>SMLKLSAENESTPIQQLLEHFLRQLQRKDPHGFFAFPVTDAIAPGYSMIIKHPMDFGTMKDKIVANEYKSVTEFKADFKLMCDNAMTYNRPDTVYYKLAKKILHAGFKMMSKERLLALKRSMS[2x]

Bromodomains (BRDs) are acetyl-lysine–dependent protein interaction modules that play a pivotal role in chromatin biology and control of gene expression. Acetyl-lysine recognition is mediated by a binding cleft formed by four canonical helices (αZ, αA, αB, and αC) and two connecting loop regions (ZA and BC loops). This interaction site is highly druggable, enabling the development of potent protein interaction inhibitors. To address this issue, we developed a promiscuous BRD inhibitor [bromosporine (BSP)] that broadly targets BRDs (including BETs) with nanomolar affinity, creating a tool for the identification of cellular processes and diseases where BRDs have a regulatory function.

To ascertain the predicted promiscuous binding mode, we determined high-resolution crystal structures with different human BRDs. In all cases, BSP was resolved well in the high-resolution structures and inserted into the acetyl-lysine binding cavity of each BRD module. In all cases, BSP exhibited a common binding mode, whereby it engaged the conserved asparagine [N100 in BRD9, N140 in BRD4(1), and N1602 in TAF1L(2)] while extending its sulfonamide substituent toward the front of the ZA-loop binding cavity. The excellent shape complementarity with diverse acetyl-lysine binding sites explained its high binding potency, which we further characterized in solution by isothermal titration calorimetry (ITC). Although most BRD-containing proteins are expressed in HEK293 cells, we observed enriched binding to most high-affinity in vitro targets of BSP and also identified binding partners from larger complexes, such as the SWI/SNF BRD-containing proteins SMARCA2/SMARCA4 and PB1, which were most likely enriched as a result of a tight interaction with the BSP targets BRD7/BRD9 (22). We used a fluorescence recovery after photobleaching (FRAP) technique to disrupt the interaction of full-length green fluorescent protein (GFP)–tagged BRD4 or full-length GFP-tagged BRD9 with acetylated chromatin. In both cases, we observed displacement of proteins from chromatin, as evidenced by the fast recovery after bleaching. In the case of BRD9, we treated cells with the histone deacetylase inhibitor SAHA (suberoylanilide hydroxamic acid) to increase acetylation levels and to enhance binding.>[2x]MVPISPIETVPVKLKPGMDGPKVKQWPLTEEKIKALVEICTEMEKEGKISKIGPENPYNTPVFAIKKKDSTKWRKLVDFRELNKRTQDFWEVQLGIPHPAGLKKK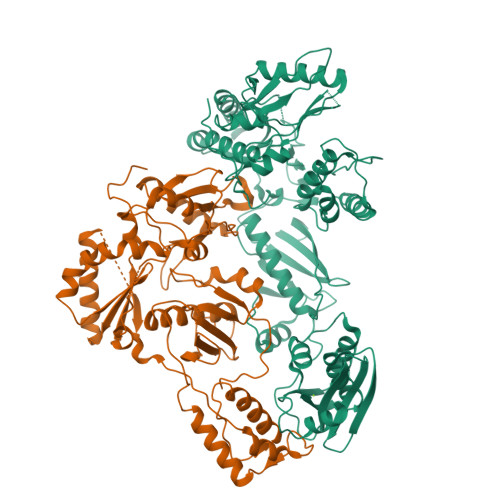KSVTVLDVGDAYFSVPLDEDFRKYTAFTIPSINNETPGIRYQYNVLPQGWKGSPAIFQSSMTKILEPFKKQNPDIVIYQYMDDLYVGSDLEIGQHRTKIEELRQHLLRWGLTTPDKKHQKEPPFLWMGYELHPDKWTVQPIVLPEKDSWTVNDIQKLVGKLNWASQIYPGIKVRQLSKLLRGTKALTEVIPLTEEAELELAENREILKEPVHGVYYDPSKDLIAEIQKQGQGQWTYQIYQEPFKNLKTGKYARMRGAHTNDVKQLTEAVQKITTESIVIWGKTPKFKLPIQKETWETWWTEYWQATWIPEWEFVNTPPLVKLWYQLEKEPIVGAETFYVDGAANRETKLGKAGYVTNKGRQKVVPLTNTTNQKTELQAIYLALQDSGLEVNIVTDSQYALGIIQAQPDKSESELVNQIIEQLIKKEKVYLAWVPAHKGIGGNEQVDKLVSAG;>[2x]GPISPIETVPVKLKPGMDGPKVKQWPLTEEKIKALVEICTEMEKEGKISKIGPENPYNTPVFAIKKKDSTKWRKLVDFRELNKRTQDFWEVQLGIPHPAGLKKKKSVTVLDVGDAYFSVPLDEDFRKYTAFTIPSINNETPGIRYQYNVLPQGWKGSPAIFQSSMTKILEPFKKQNPDIVIYQYMDDLYVGSDLEIGQHRTKIEELRQHLLRWGLTTPDKKHQKEPPFLWMGYELHPDKWTVQPIVLPEKDSWTVNDIQKLVGKLNWASQIYPGIKVRQLSKLLRGTKALTEVIPLTEEAELELAENREILKEPVHGVYYDPSKDLIAEIQKQGQGQWTYQIYQEPFKNLKTGKYARMRGAHTNDVKQLTEAVQKITTESIVIWGKTPKFKLPIQKETWETWWTEYWQATWIPEWEFVNTPPLVKLWYQ> MGRTANILKPLMSPP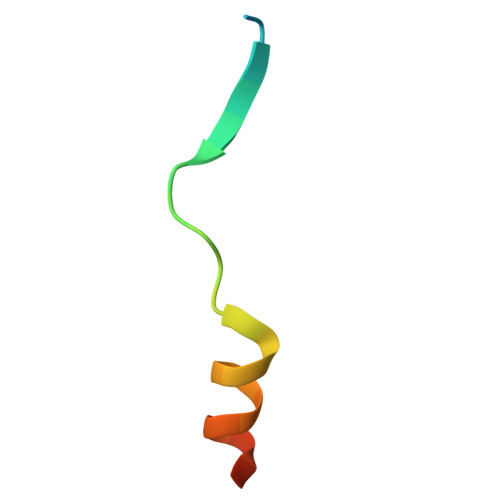SREEIMATLLDHD>[4x]GSLGKRPDAVSQAVSSLQGLSPEQADLVAKLKNGHLSERVLAANKLRFAVVDFPLNPVHAIW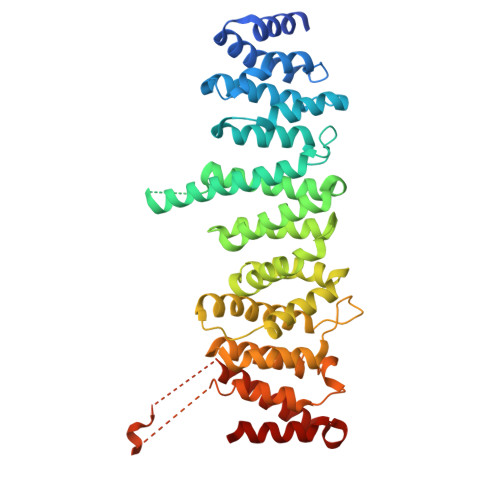HAAKDMIHPENPDNARQASWELLIECVKYPNSTELERSEYFHTLTGPAHSKDFCYQLVALEQLTNHGRNIAGFYYEMFPLLTLWLNQAYRAARDARKLALARGATKNSSKGKAPASPEDKNLSQLFALVKDVIKFNFKFATDDVIAGLIDMLLKICMLTSVEDDLRACIHVIESLVTFGSIPTNKLKYCIQVLSSIHCLVPSLQKEAWHTISIICRSHHGQSTVRILLDFLRSYSPNPDKNREKDTVRDVRGALSVLQKLLRKTAEKGYPQVPLSLLVGGLANVSKSSSTRVATEILRLINSLFHGREGNINPILVEEHWEPIFDVAAQCATKAVTLPPADASASPLPTVAKEEPVVEDNVSLQLKHLILRVENLIVHQGPELLQRDDCMKFLIRVQHALP2'-((5-CARBAMIMIDOYLPYRIDIN-2-YLAMINO)METHYL)-4-(ISOBUTYLCARBAMOYL)-4'-VINYLBIPHENYL-2-CARBOXYLIC ACID | C27 H29 N5 O3 | 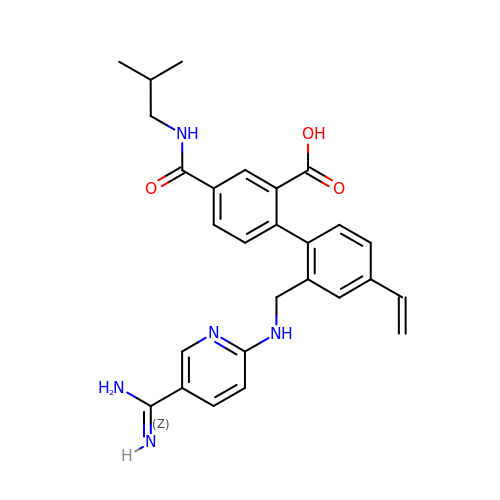HHFWQMFTPDFWLM-UHFFFAOYSA-N The eukaryotic guided entry of tail-anchored proteins (GET) pathway mediates the biogenesis of tail-anchored (TA) membrane proteins at the endoplasmic reticulum. In the cytosol, the Get3 chaperone captures the TA protein substrate and delivers it to the Get1/Get2 membrane protein complex (GET insertase), which then inserts the substrate via a membrane-embedded hydrophilic groove. Within the membrane targeting stages of the GET pathway, the homodimeric ATPase Get3 (also called TRC40 in metazoans) adopts closed and open conformations in response to nucleotide load and interactions with other pathway components, allowing binding and release of the TA protein respectively. However, the cryo-EM structures and native mass spectrometry of hsGet1/Get2 and scGet1/Get2 show they form a 2:2 heterotetramer, which is stabilised by Get3 and interfacial lipid binding and is important for efficient TA protein insertion.

We subsequently obtained single-particle cryo-EM reconstructions of both amphipol- and nanodisc-reconstituted ctGet2ΔN-Get1/Get3 at an overall resolution of 5.0 Å and 4.6 Å respectively. In both reconstructions, there is clear density in the membrane region for two three-helix bundles at a local resolution of 6.5 Å. Weak density also shows that helix α3’ is present in the same conformation relative to ctGet2 TMD3 in both the amphipol and nanodisc reconstruction. Furthermore, the density map for the nanodisc-reconstituted sample provides evidence that ctGet2 TMD1 and TMD2 occupy the same position in the heterodimer as the equivalent hsGet2 TMDs, albeit they are poorly resolved and likely exhibit flexibility on the edge of the complex. Interestingly, the conserved fold of the ctGet1/Get2 heterodimer adopts a different position in the membrane compared to the structure of hsGet1/Get2, with each heterodimer half exhibiting a 40° rotation with respect to the membrane plane. This is largely due to ctGet1 TMD1/TMD2 not adopting the parallel arrangement observed for hsGet1, instead being tilted by 40° relative to each other. As a result of the rearrangement of ctGet1/Get2, the hydrophilic groove of ctGet1/Get2 is tilted so that it is open towards the cytosolic leaflet of the membrane, in contrast to the hsGet1/Get2 hydrophilic groove opening to the cytosol. In addition, ctGet2 TMD3 no longer completely traverses the ER membrane, which is notable given the high number of charged residues found at the N-terminal portion of this helix and the adjoining cytoplasmic loop. Indeed, we observe significant thinning of the nanodisc in the vicinity of ctGet2 TMD3. As this helix encloses one side of the hydrophilic groove, such membrane distortion would likely lower the energetic barrier for substrate insertion.

>[2x]MEPTLQSILDQRSLRWIFVGGKGGVGKTTTSCSLAIQLAKVRRSVLLLSTDPAHNLSDAFSQKFGKEARLVEGFDNLYAMEIDPNGSMQDLLAGQTGDGDAGMGGVGVMQDLAYAIPGIDEAMSFAEVLKQVNSLSYETIVFDTAPTGHTLRFLQFPTVLEKALAKVSQLSGQYGSLLNGILGGSGTLPNGQTLSDVMEKLDSLRVTISEVNAQFKDERLTTFVCVCIPEFLSLYETERMIQELANYGIDTHCIVVNQLLFPKPGSDCEQCTARRRMQKKYLDQIEELYDEEFNVVKMPLLVEEVRGKERLEKFSEMLIKPFVPPEWSHPQFEK;>[2x]MGRPTPLWRFLHTLLAVALGLAVIMLSPFGGTKLERDRAAAAVAGSASEREWLASLTDSYPLVKTGLGGGLFWAFATGEAILLGTRWLFLSKKKKAATAAAKVNNNNGEGDDAELDSVEQAIELALEFFPAIRQPVEYLRPKVAVAMRYVDVGMTLWRDVMLALFVLGAVAWWRAGSGSENLYFQSGSGSMSLLLVIFLLELVVQLVNTIGAKTINNLLWRFYLSIPGSPLAKDFAEQRAKQKEYLQVRHDLNATSSQDEFAKWARLQRKHDKLMDELEKKKSQLDAHRTSFSRKLTIYRWILTRGMQWFLCFWFSSQPMFWLPYGWFPYWVEWLVSFPNAPMGSVSIVVWQSACSGVLALVIEAVMAVVRYTGGTGMQKQRQPVPAAGGAPGTSKKDLGSGSLEVLFQ>[3x]SVRSSSRTPSDKPVAHVVANPQAEGQLQWLNRRANALLANGVELRDNQLVVPSEGLYLIYSQVLFKGQGCPSTHVLLTHTISRIAVSYQTKVNLLSAIKSPCQRETPEGAEAKPWYEPIYLGGVFQLEKGDRLSAEINRPDYLDFAESGQVYFGIIAL

TNF, like most members of the TNF superfamily (TNFSF) exists mainly as a trimer with a threefold symmetry resulting in three identical receptor binding sites. The mechanism by which TNF induces signalling across the membrane is poorly understood, however, it is generally believed that the process involves receptor clustering. There are currently five approved TNF biologics that work by completely blocking the interaction of TNF with its receptors but to date, there are no small molecule therapeutics available that disrupt the high-affinity TNF–TNFR interaction. Small molecule inhibitors of TNF are described that stabilise a distorted TNF trimer, reducing the affinity of TNFR1 at one binding site and effectively reducing the stoichiometry of receptor binding from three to two per TNF trimer.

Recently, we described small molecule inhibitors of TNF that stabilised a distorted conformation of human TNF (hTNF) by binding in a pocket within the trimer core. Each of the compounds bound hTNF in a similar mode within the trimer core, resulting in an equivalent degree of distortion in the trimer. In order to strengthen the correlation between structural observations made with the mTNF(UCB-4433)–TNFR1 complex and how they are likely to also apply to hTNF, a comparison of the binding mode of UCB-4433 in human and mouse TNF was made.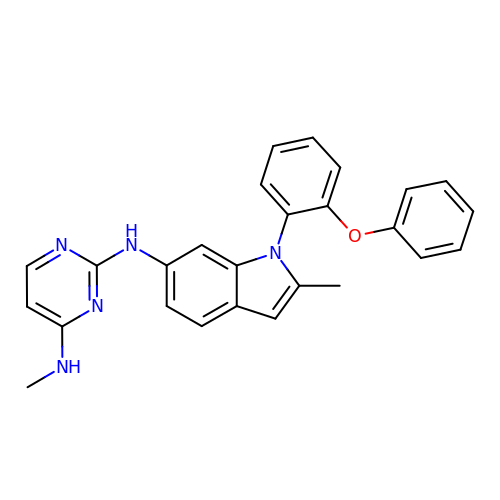N~4~-methyl-N~2~-[2-methyl-1-(2-phenoxyphenyl)-1H-indol-6-yl]pyrimidine-2,4-diamine | C26 H23 N5 O | VTOOSSZNUMLKNN-UHFFFAOYSA-N> MASTGETTYKKTTSSALKGAIQLGITHSVGSLSQKPERDVLMQDFEVVESIFFPSQGSSSTPGHHHGDFKFKTYAPIAFRYFREMFGIRPDDYLYSLCNEPLIELSNPGASGSLFYVSSDDEFIIKTVQHKEAEFLQTLLPGYFMNLNQNMRTLLPKFYGLYCVQADGKNIRIVVMNNLLPRAVPMHLKFALKGSTYKRRASPKERSKGVPTYKDLDFMQDMPEGILLENDHYTALSRTMQRDCRVLQSFKIMDYSLLVGIHILHRAGEEASTAVPDTQKKGQGQKPLYCTAIESIQGESKSKTSPQPYESMGGIPAFNSKGERLLVFIGIIDILQSYRL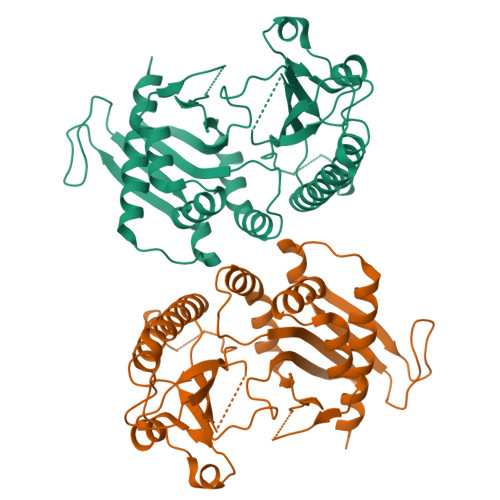VKKLEHSWKALLHDGDTVSVHRPSFYADRFQKFMCSTVFRKSQLKTLEHHHHHH>[2x]MAHHHHHHMSYSKIPAGKDLPNDIYVAIEIPANHAPIKYEIDKDTDCLFVDRFMATPMFYPANYGFIPNTLADDGDPLDVLVVTPYPVAPGSVIRARPVGVLHMT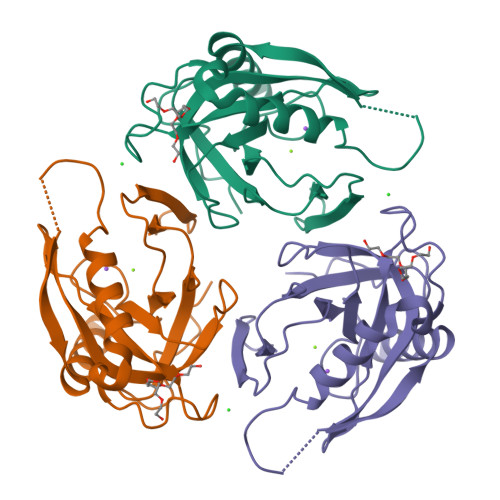DEAGGDAKLIAVPHDKLSVLYKDVKEYTDLPALLLEQIKHFFENYKDLEKGKWVKVEGWGNADAARAEITKAVAAFQK>MSREEVESLIQEVLEVYPEKARKDRNKHLAVNDPAVTQSKKCIISNKKSQPGLMTIRGCAYAGSKGVVWGPIKDMIHISHGPVGCGQYSRAGRRNYYIGTTGVNAFVTMNFTSDFQEKDIVFGGDKKLAKLIDEVETLFPLNKGISVQSECPIGLIGDDIESVSKVKGAELSKTIVPVRCEGFRGVSQSLGHHIANDAVRDWVLGKRDEDTTFASTPYDVAIIGDYNIGGDAWSSRILLEEMGLRCVAQWSGDGSISEIELTPKVKLNLVHCYRSMNYISRHMEEKYGIPWMEYNFFGPTKTIESLRAIAAKFDESIQKKCEEVIAKYKPEWEAVVAKYRPRLEGKRVMLYIGGLRPRHVIGAYEDLGMEVVGTGYEFAHNDDYDRTMKEMGDSTLLYDDVTGYEFEEFVKRIKPDLIGSGIKEKFIFQKMGIPFREMHSWDYSGPYHGFDGFAIFARDMDMTLNNPCWKKLQAPWE[2x];>SQQVDKIKASYPLFLDQDYKDMLAKKRDGFEEKYPQDKIDEVFQWTTTKEYQELNFQREALTVNPAKACQPLGAVLCALGFEKTMPYVHGSQGCVAYFRSYFNRHFREPVSCVSDSMTEDAAVFGGQQNMKDGLQNCKATYKPDMIAVSTTCMAEVIGDDLNAFINNSKKEGFIPDEFPVPFAHTPSFVGSHVTGWDNMFEGIARYFTLKSMDDKVVGSNKKINIVPGFETYLGNFRVIKRMLSEMGVGYSLLSDPEEVLDTPADGQFRMYAGGTTQEEMKDAPNALNTVLLQPWHLEKTKKFVEGTWKHEVPKLNIPMGLDWTDEFLMKVSEISGQPIPASLTKERGRLVDMMTDSHTWLHGKRFALWGDPDFVMGLVKFLLELGCEPVHILCHNGNKRWKKAVDAILAASPYGKNATVYIGKDLWHLRSLVFTDKPDFMIGNSYGKFIQRDTLHKGKEFEVPLIRIGFPIFDRHHLHRSTTLGYEGAMQILTTLVNSILERLDEETRGMQATDYNHDLVR[2x];> MSWRILLCHKHPVSARLRFLIPTGGGVVLPQTLPRLAVIAEDQEAPVQCHPASALRALQETMALGWQLELIGEFRLNMEVPGQIMPIYLAALAGHELPPPPEGTRWIELTQSIGMPWLDRELLRRVYEELIG

Nitrogenase catalyzes the ATP-dependent reduction of dinitrogen to ammonia during the process of biological nitrogen fixation that is essential for sustaining life. The Fe-protein mediates ATP-dependent electron transfer (ET) through its [4Fe:4S] cluster to the intermediate [8Fe:7S] P-cluster in the MoFe-protein; the electrons are subsequently shuttled to a [7Fe:1Mo:9S:1C]-R-homocitrate metallocluster, the FeMo-cofactor, within the active site of the MoFe-protein. The active site FeMo-cofactor contains a [7Fe:1Mo:9S:1C] metallocluster coordinated with an R-homocitrate (HCA) molecule.

Further data collection and classification of a subset of MoFeΔNifV particles resulted in a 2.71 Å overall resolution map with a protruding density that we hypothesized belonged to an endogenous binding partner pulled down with MoFeΔNifV during purification. A partial model built into this additional density was cross-referenced against Alpha Fold-predicted models of proteins identified in purified MoFeΔNifV samples by proteomic analysis. This approach revealed that the AlphaFold model of an uncharacterized protein of 15 kDa, a product of the Avin_01560 gene on the nif operon, matched the extended density. Building the model into this density yields the MoFeΔNifV-NafT complex. The binding site for this protein on MoFeΔNifV partially overlaps with that of the nitrogenase Fe-protein in the MoFe-protein:Fe-protein ADP-AlF4- stabilized complex and buries approximately ~1,400 Å2 surface area (PDB 1N2C38). At the interface between the two proteins, a well-ordered amphipathic helix from Trp ε117 to Ile ε131 packs against the MoFeΔNifV protein α- and β-subunits. Additionally, a loop in NafT spanning residues Lys ε10 to Leu ε17 extends into the MoFeΔNifV α-subunit. This extension allows for hydrogen bonding between Ser ε14 and Tyr α281, and a salt bridge between Arg ε16 and Asp α200. Perhaps more strikingly, this loop adds two histidines (His ε9 and His ε11) to a cluster of histidines that includes His ε95, His α195, and His α196, four of which are situated within 10 Å of each other. In the MoFeΔNifV-NafT state, the MoFeΔNifV shows asymmetric disordering of residues 1–48, 376–383, 390–398, and 402–409 in one of its α-subunits.> GSGGSGGITEAQARAIVNSALKLYSQDKTGMVDFALESGGGSILSTRCSETYETKTALMSLFGIPLWYFSQSPRVVIQPDIYPGNCWAFKGSQGYLVVRLSMMIHPAAFTLEHIPKTLSPTGNISSAPKDFAVYGLENEYQEEGQLLGQF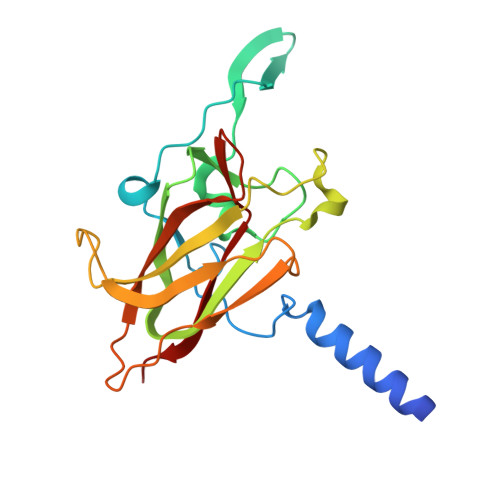TYDQDGESLQMFQALKRPDDTAFQIVELRIFSNWGHPEYTCLYRFRVHGEPVK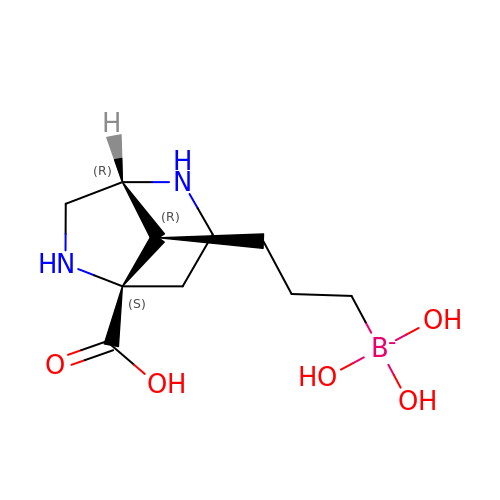3-[(1~{R},5~{S},8~{R})-5-carboxy-2,6-diazabicyclo[3.2.1]octan-8-yl]propyl-$l^{3}-oxidanyl-bis(oxidanyl)boranuide | C10 H20 B N2 O5 | LAVGLMPTAZJTQK-WEDXCCLWSA-N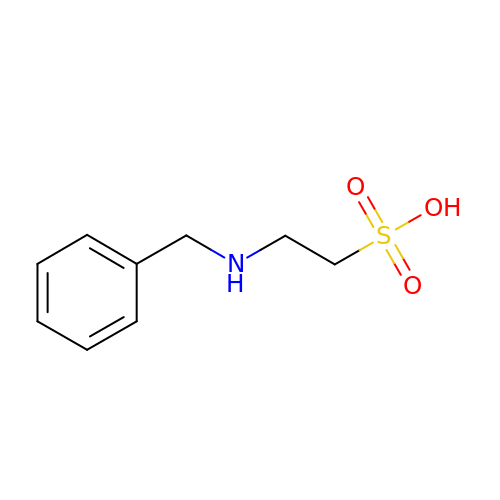2-(benzylamino)ethanesulfonic acid | C9 H13 N O3 S | DRWVGXPRVWLEPQ-UHFFFAOYSA-N>[2x]MWRKLLNNHHDDASKFICLLAKPNCSSLEQEDFIPLLQDVVDTHPGLTFLKDAPEFHSRYITTVIQRIFYTVNRSWSGKITSTEIRKSNFLQTLALLEEEEDINQITDYFSYEHFYVIYCKFWELDTDHDLYISQADLSRYNDQASSSRIIERIFSGAVTRGKTIQKEGRMSYADFVWFLISEEDKRNPTSIEYWFRCMDVDGDGV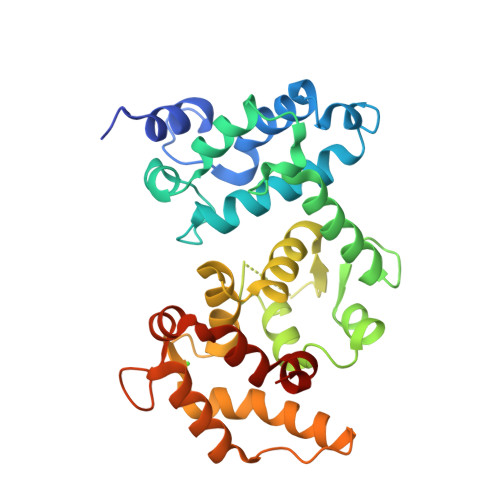LSMYELEYFYEEQCERMEAMGIEPLPFHDLLCQMLDLVKPAVDGKITLRDLKRCRMAHIFYDTFFNLEKYLDHEQRDPF> SIPTVERSTRMSNPWKAFMEKYDIERTHSSGVRVDLGEDAEVENAKYRIPAGRCPVFGKGIVIENSDVSFLRPVATGDQKLKDGGFAFPNANDHISPMTLANLKERYKDNVEMMKLNDIALCRTHAASFVMAGDQNSNYRHPAVYDEKEKTCHMLYLSAQENMGPRYCSPDAQNRDAVFCFKPDKDESFENLVYLSKNVRNDWDKKCPRKNLGNAKFGLWVDGNCEEIPYVKEVEAEDLRECNRIVFGASASDQPTQYEEEMTDYQKIQQGFRQNNREM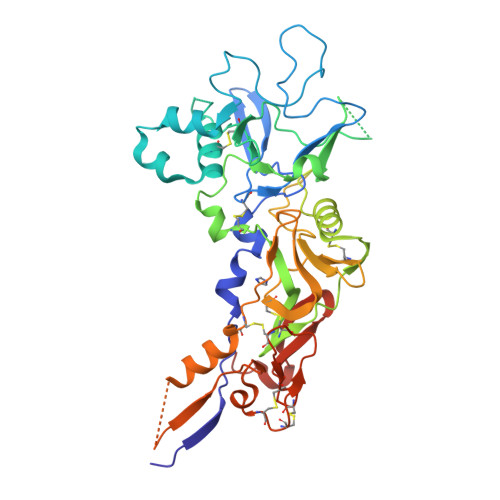IKSAFLPVGAFNSDNFKSKGRGFNWANFDSVKKKCYIFNTKPTCLINDKNFIATTALSHPQEVDLEFPCSIYKDEIEREIKKQSRNMNLYSVDGERIVLPRIFISNDKESIKCPCEPERISQSTCNFYVCNCVEKRAEIKENNQVVIKEEFRDYYENGEEKSNKQMLL> AGAGAAGAUCUUCUCU

Since DNA/RNA duplexes are known to be less stable than RNA/RNA duplexes, we have examined the impact of dA, dI, and dG substitutions on RNA structure and nonenzymatic template copying. In this study, we have investigated the effects of 2′-deoxyribo-purines on nonenzymatic template copying by conducting thermodynamic, structural, and kinetic analyses. Structural analyses of RNA duplexes containing 2′-deoxyribo-purine nucleotides suggest that the observed destabilization is likely due to reduced solvation effects, since base pairing and sugar conformations are unchanged. Our results suggest that a primordial genetic polymer containing both ribo- and 2′-deoxyribo- nucleotides would likely behave similarly to RNA but with somewhat slower template copying chemistry, offset by a possible advantage in strand separation and exchange, which could in turn facilitate cycles of replication.

Among these, four sequences (dAU1, dAU2, dAUS1, and dAUS2) contained base pairs involving deoxyadenosine (dA:U and dA:s2U), four (dGC1, dGC2, dGCS1, and dGCS2) contained deoxyguanosine base pairs (dG:C and dG:s2C), and two (dICS1 and dICS2) included base pairs with deoxyinosine (dI:s2C). Eight of the ten structures crystallized in the same space group (H32) with similar packing, each unit cell containing a single RNA strand. When paired with the same pyrimidines, including 2-thiopyrimidines, ribo- and deoxyribo-purines formed the same number of hydrogen bonds with similar bond lengths. Additionally, the introduction of a single deoxyribo-purine modification into RNA duplexes did not result in any detectable perturbation of the local sugar pucker conformation or the overall helical geometry. Due to the absence of the 2′-hydroxyl group, the 2′-deoxyribose sugars exhibit fewer hydrogen bonding interactions with surrounding solvent molecules. Base pairs involving deoxyadenosine (dA) and deoxyinosine (dI), especially those paired with 2-thiopyrimidines (dA:s2U and dI:s2C), exhibit enthalpic penalties accompanied by entropic gains, relative to their ribonucleotide counterparts (A:s2U and I:s2C). The net effect is a ΔG°25°C penalty of ~1.2–1.4 kcal/mol. Due to their similar thermodynamic trends and compensatory changes, dA:s2U and dI:s2C, like A:s2U and I:s2C, are essentially isoenergetic. The dA:s2U pair is only marginally more stable than the s2U:s2U mismatch, with a ΔG°25°C difference of just 0.6 kcal/mol.> AKPVWAPHPTDGFQVGNIVDIGPDSLTIEPLNQKGKTFLALINQVFPAEEDSKKDVEDNCSLMYLNEATLLHNIKVRYSKDRIYTYVANILIAVNPYFDIPKIYSSETIKSYQGKSLGTMPP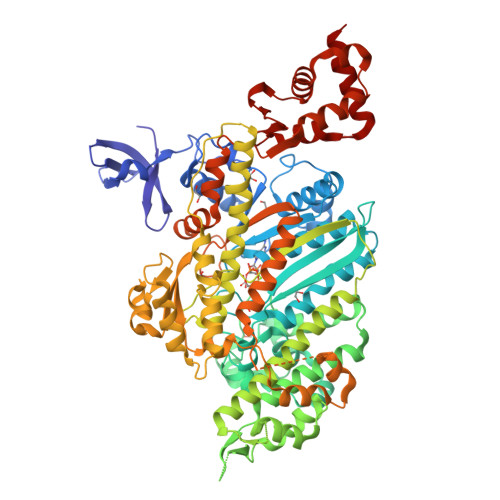HVFAIADKAFRDMKVLKLSQSIIVSGESGAGKTENTKFVLRYLTESYGTGQDIYDRIVEANPLLEAFGNAKTVRNNNSSRFGKFVEIHFNEKSSVVGGFVSHYLLEKSRICVQGKEERNYHIFYRLCAGASEDIRERLHLSSPDNFRYLNRGCTRYFANKETDKQILQNRKSPEYLKAGSLKDPLLDDHGDFIRMCTAMKKIGLDDEEKLDLFRVVAGVLHLGNIDFEEAGSTSGGCNLKNKSTQALEYCAELLGLDQDDLRVSLTTRVMLTTAGGAKGTVIKVPLKVEQANNARDALAKTVYSHLFDHVVNRVNQCFPFETSSYFIGVLDIAGFEYFEHNSFEQFCINYCNEKLQQFFNERILKEEQELYQKEGLGVNEVHYVDNQDCIDLIEARLVGILDILDEENRLPQPSDQHFTSAVHQKHKDHFRLSIPRKSKLAIHRNIRDDEGFIIRHFAGAVCYETTQFVEKNNDALHMSLESLICESRDKFIRELFESSTNNNKDTKQKAGKLSFISVGNKFKTQLNLLLDKLRSTGASFIRCIKPNLKMTSHHFEGAQILSQLQCSGMVSVLDLMQGGFPSRASFHELYNMYKKYMPDKLARLDPRLFCKALFKALGLNEIDYKFGLTKVFFRPGKFAEFDQIMKSDPDHLAELVKRVNHWLI>[4x]MPGFYEI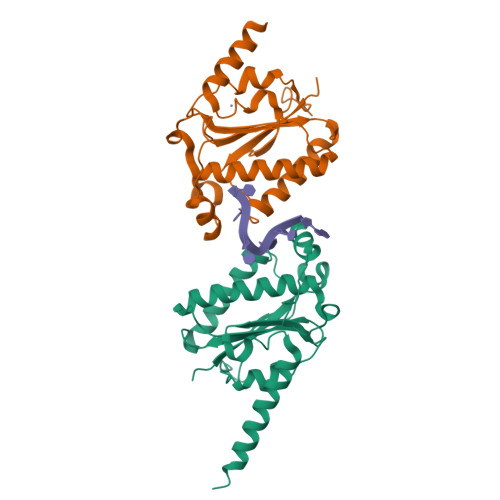VIKVPSDLDEHLPGISDSFVNWVAEKEWELPPDSDMDLNLIEQAPLTVAEKLQRDFLTEWRRVSKAPEALFFVQFEKGESYFHMHVLVETTGVKSMVLGRFLSQIREKLIQRIYRGIEPTLPNWFAVTKTRNGAGGGNKVVDESYIPNYLLPKTQPELQWAWTNMEQYLSACLNLTERKRLVAQHLTHVSQTQEQNKEN> MVSAIKPDMRIKLRMEGNVNGHHFVIDGDGTGKPYEGKQTMDLEVKEGGPLPFAFDILTTAFHYGNRVFVKYPDNIQDYFKQSFPKGYSWERSLTFEDGGICNARNDITMEGDTFYNKVRFYGTNFPANGPVMQKKTLKWEPSTEKMYVRDGVLTGDIEMALLLEGNAHYRCDFRTTYKAKEKGVKLPGAHFVDHAIEILS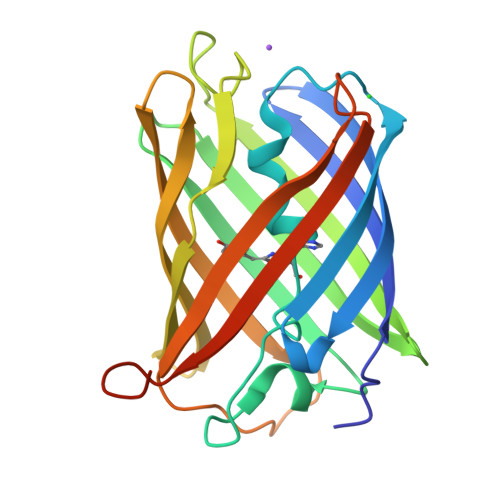HDKDYNKVKLYEHAVAHSGLPDNARRGSHHHHHH>[2x]ADKELKFLVVDDFSTMRRIVR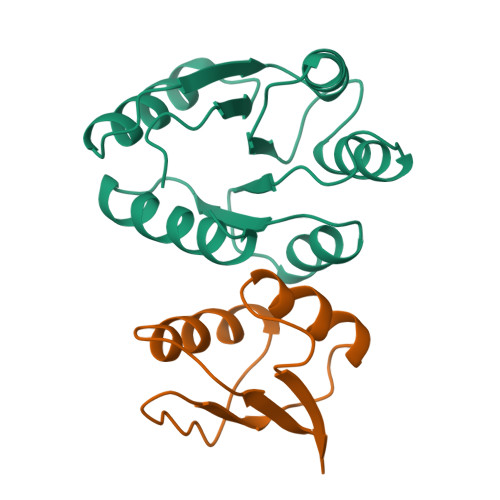NLLKELGFNNVEEAEDGVDALNKLQAGGYGFVISDWNMPNMDGLELLKTIRADGAMSALPVLMVTAEAKKENIIAAAQAGASGYVVKPFTAATLEEKLNKIFEKLGM;>[2x]MSQSPRRIILSRLKAGEVDLLEEELGHLTTLTDVVKGADSLSAILPGDIAEDDITAVLCFVIEADQITFETVEV>[2x]QDSLSFGFPTFPSDQKNLIFQGDAQIKNNAVQLTKTDSNGNPVASTVGRILFSAQVHLWEKSSSRVANFQSQFSFSLKSPLSNGADGIAFFIAPPDTTIPSGSGGGLLGLFAPGTAQNTSANQVIAVEFDTFYAQDSNTWDPNYPHIGIDVNSIRSVKTVKWDRRDGQSLNVLVTFNPSTRNLDVVATYSDGTRYEVSYEVDVRSVLPEWVRVGFSAASGEQYQTHTLESWSFTSTLLY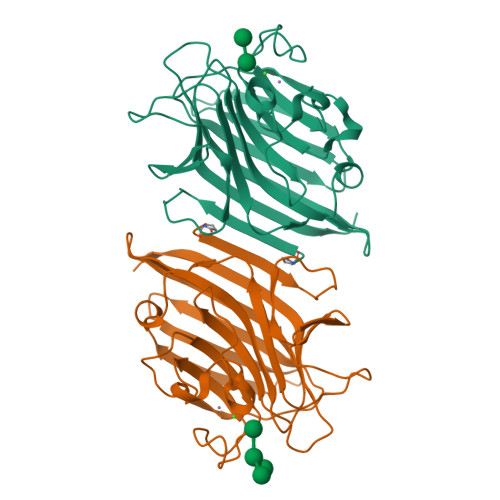TAQKKGENLALEM> VVT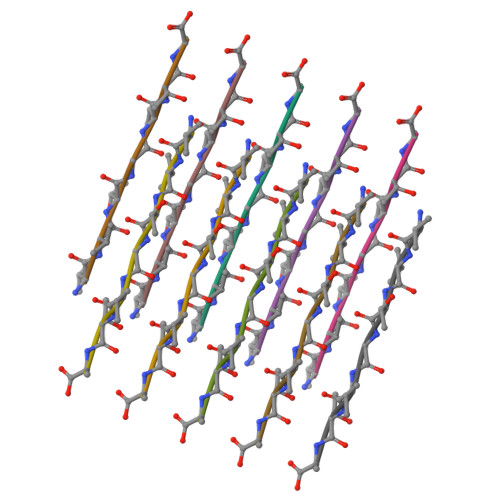GVTA> GDPVEDIIHDALSSTVRRAITSGQDVNTAAGTAPSSHRLETGRVPALQAAETGATSNATDENMIETRCVMNRNGVLEATISHFFSRSGLVGVVNLTDGGTDTTGYAVWDIDIMGFVQLRRKCEMFTYMRFNAEFTFVTTTENGEARPFMLQYMYVPPGAPKPTGRDAFQWQTATNPSVFVKLTDPPAQVSVPFMSPASAYQWFYDGYPTFGQHPETSNTTYGQCPNNMMGTFAVRVV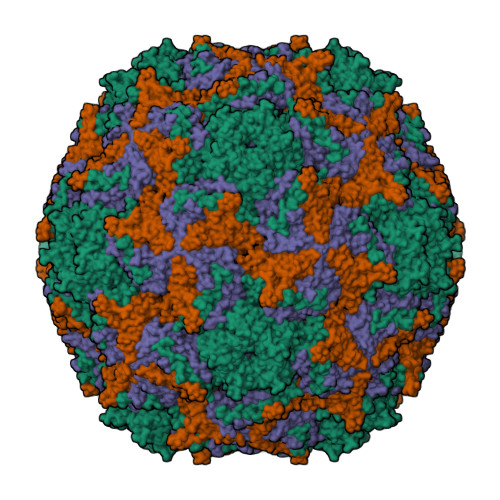SRVASQLKLQTRVYMKLKHVRAWIPRPIRSQPYLLKNFPNYDSSKITYSARDRASIKQANM;> SPSVEACGYSDRVAQLTVGNSSITTQEAANIVLAYGEWPEYCPDTDATAVDKPTRPDVSVNRFYTLDSKMWQENSTGWYWKFPDVLNKTGVFGQNAQFHYLYRSGFCLHVQCNASKFHQGALLVAVIPEFVLAGRGSNTKPNEAPHPGFNTTFPGTAGASFNDPYVLDSGVPLSQSLIYPHQWINLRTNNCATIIVPYINAVPFDSAINHSNFGLIVVPVSPLKYSSGATTAIPITVTIAPLNSEFGGLRQAVSQ;> GLPTELRPGTNQFLTTEDDTAAPILPGFSPTPSIHIPGEVRSLLELCRVETILEVNNTTDATGLNRLLIPVSAQNKADELCAAFMVDPGRIGPWQSTLVGQICRYYTQWSGSLKVTFMFTGSFMATGKMLIAYSPPGSAQPANRETAMLGTHVIWDFGLQSSVSLVIPWISNTHFRTAKTGGNYDYYTAGVVTLWYQTNYVVPPETPGEAYIIAMGAAQDNFTLKICKDTDEVTQQAVLQ>EAPYASLTEIEHLVQSVCKSYRETCQLRLEDLLRQRSNIFSREEVTGYQRKSMWEMW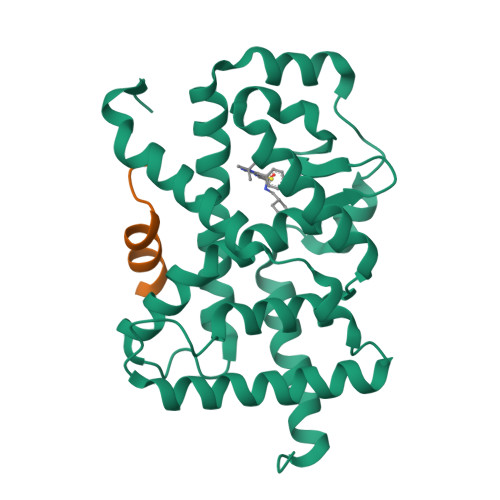ERCAHHLTEAIQYVVEFAKRLSGFMELCQNDQIVLLKAGAMEVVLVRMCRAYNADNRTVFFEGKYGGMELFRALGCSELISSIFDFSHSLSALHFSEDEIALYTALVLINAHRPGLQEKRKVEQLQYNLELAFHHHLCKTHRQSILAKLPPAGKLASLCSQHVERLQIFQHLHPIVVQAAFPPLYKELFSTETESPVGLSK[4x];>TNMGLEAIIRKALMGKYDQWEE[4x]>[2x]MESLASLYKNHIATLQERTRDALARFKLDALLIHSGELFNVFLDDHPYPFKVNPQFKAWVPVTQVPNCWLLVDGVNKPKLWFYLPVDYWHNVEPLPTSFWTEDVEVIALPKADGIGSLLPAARGNIGYIGPVPERALQLGIEASNINP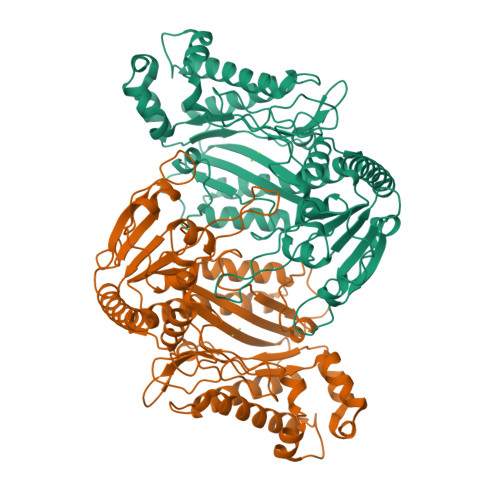KGVIDYLHYYRSFKTEYELACMREAQKMAVNGHRAAEEAFRSGMSEFDINIAYLTATGHRDTDVPYSNIVALNEHAAVLHYTKLDHQAPEEMRSFLLDAGAEYNGYAADLTRTWSAKSDNDYAQLVKDVNDEQLALIATMKAGVSYVDYHIQFHQRIAKLLRKHQIITDMSEEAMVENDLTGPFMPHGIGHPLGLQVHDVAGFMQDDSGTHLAAPAKYPYLRCTRILQPGMVLTIEPGIYFIESLLAPWREGQFSKHFNWQKIEALKPFGGIRIEDNVVIHENNVENMTRDLKLA>RTIVVTTILESPYVMYKKNHEQLEGNERYEGYCVDLAYEIAKHVRIKYKLSIVGDGKYGARDPETKIWNGMVGELVYGRADIAVAPLTITLVREEVIDFSKPFMSLGISIMIKKGTPIESAEDLAKQTEIAYGTLDSGSTKEFFRRSKIAVYEKMWSYMKSAEPSVFTKTTADGVARVRKSKGKFAFLLESTMNEYIEQRKPCDTMKVGGNLDSKGYGVATPKGSALGNAVNLAVLKLNEQGLLDKLKNKWWYDKGEC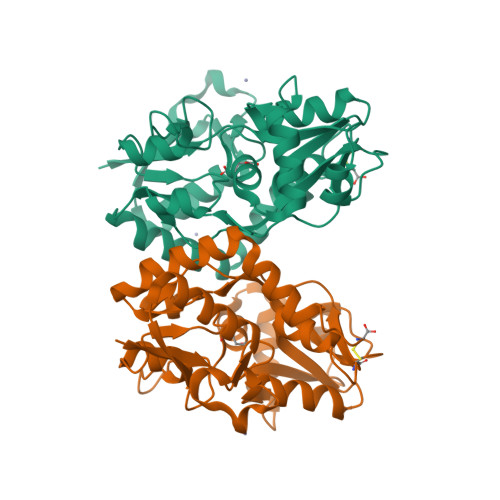[3x]>HFLCGVVEGFYGRPWVMEQRKELFRRLQKWELNTYLYAPKDDYKHRMFWREMYSVEEAEQLMTLISAAREYEIEFIYAISPGLDITFSNPKEVSTLKRKLDQVSQFGCRSFALLFDNIDHNMCAADKEVFSSFAHAQVSITNEIYQYLGEPETFLFCPTEYCGTFCYPNVSQSPYLRTVGEKLLPGIEVLWTGPKVVSKEIPVESIEEVSKIIKRAPVIWDNIHANDYDQKRLFLGPYKGRSTELIPRLKGVLTNPNCEFEANYVAIHTLATWYKSNMNGVRKDVVMTDSEDSTVSIQIKLENEGSDEDIETDVLYSPQMALKLALTEWLQEFGVPHQYSSRGGGGSGGGGSVTLEDLQLLADLFYLPYEHGPKGAQMLREFQWLRANSSVVSVNCKGKDSEKIEEWRSRAAKFEEMCGLVMGMFTRLSNCANRTILYDMYSYVWDIKSIMSMVKSFVQWLGCRSHSSAQFLIGDQEPWAFRGGLAGEFQRLLPIDGANDLFFQ[2x];>KLSPSPSSRVTVS[2x]

OGA is the unique enzyme responsible for O-GlcNAc hydrolysis from a large number of cytoplasmic and nuclear proteins. Recently, our group and others have independently identified crystallizable constructs of OGA that comprise the catalytic domain and stalk domain, and published the apo form structures and enzyme complexes with active site inhibitors. These reports consistently showed that OGA formed an unusual arm-in-arm homodimer, where the catalytic domain of one monomer covered by the stalk domain of the sister monomer to create a potential substrate-binding cleft. Exploiting our previously reported construct of OGAcryst (residues 60–704 with the unstructured insert residues 401–552 replaced by a glycine–serine (GS) linker), we solved the structures of a mutant OGAcryst-D175N (catalytically impaired but retaining the ability to bind substrate) in apo form and in complex with each of four synthetic glycopeptides.

In the substrate complexes, all the glycopeptides were bound in the OGA substrate-binding cleft. Particularly, the GlcNAc moieties were anchored by the same set of OGA residues in the catalytic pocket, displaying nearly identical binding conformations regardless of the glycosylated residues or the flanking peptide sequences. Consistent with the O-GlcNAc hydrolysis mechanism, the catalytic residue D174 was optimally positioned to make a hydrogen bond with the N-acetyl group of GlcNAc in all the complexed structures. The N175 mutant side chain played an important role in anchoring the glycosylated hydroxyl of serine or threonine and stabilizing the OGA substrate complexes. Compared to the glycosylated serine, the extra methyl group of the glycosylated threonine (as found in ELK1 and Lamin B1 peptides in Fig. 2c, d) was well accommodated in the hydrophobic pocket harboring F223 and V254 residues from the top surface of the catalytic domain and W679 from the stalk domain of the sister monomer. Finally, in the OGA-Lamin B1 complex, the peptide was primarily stabilized by side chain specific interactions with the cleft surface residues: valine (-1 subsite) was engaged in hydrophobic and van der Waals interactions with W645, whereas arginine (-2 subsite) participated in forming a hydrogen bond with T626. We find that OGA is able to bind peptide substrates in different directions, but in a conserved conformation regardless of the glycosylation site or flanking sequences.>HMDIRTITSSDYEMVTSVLNEWWGGRQLKEKLPRLFFEHFQDTSFITSEHNSMTGFLIGFQSQSD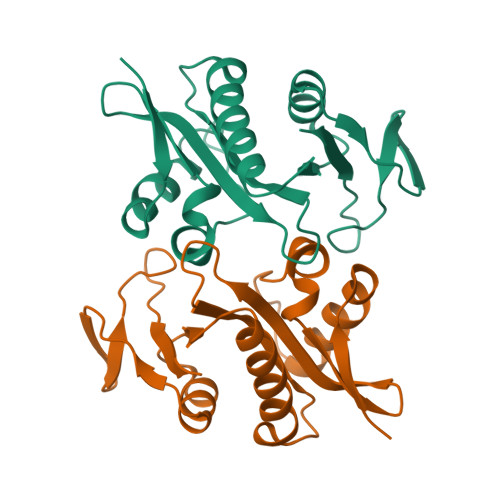PETAYIHFSGVHPDFRKMQIGKQLYDVFIETVKQRGCTRVKCVTSPVNKVSIAYHTKLGFDIEKGTKTVNGISVFANYDGPGQDRVLFVKNI[2x]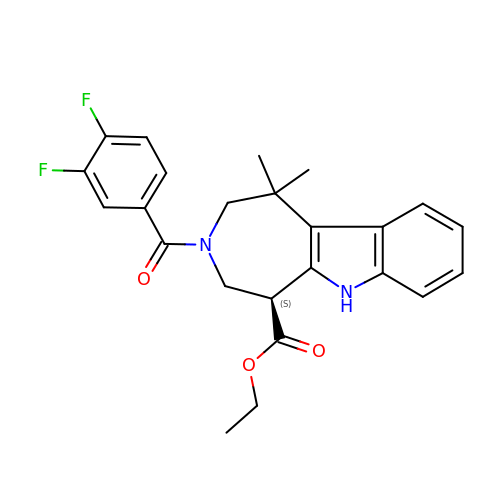ethyl (5S)-3-(3,4-difluorobenzene-1-carbonyl)-1,1-dimethyl-1,2,3,4,5,6-hexahydroazepino[4,5-b]indole-5-carboxylate | C24 H24 F2 N2 O3 | CTKZFOFWQDITSZ-INIZCTEOSA-N> MEEPEEPADSGQSLVPVYIYSPEYVSMCDSLAKIPKRASMVHSLIEAYALHKQMRIVKPKVASMEEMATFHTDAYLQHLQKVSQEGDDDHPDSIEYGLGYDCPATEGIFDYAAAIGGATITAAQCLIDGMCKVAINWSGGWHHAKKDEASGFCYLNDAVLGILRLRRKFERILYVDLDLHHGDGVEDAFSFTSKVMTVSLHKFSPGFFPGTGDVSDVGLGKGRYYSVNVPIQDGIQDEKYYQICESVLKEVYQAFNPKAVVLQLGADTIAGDPMCSFNMTPVGIGKCLKYILQWQLATLILGGGGYNLANTARCWTYLTGVILGK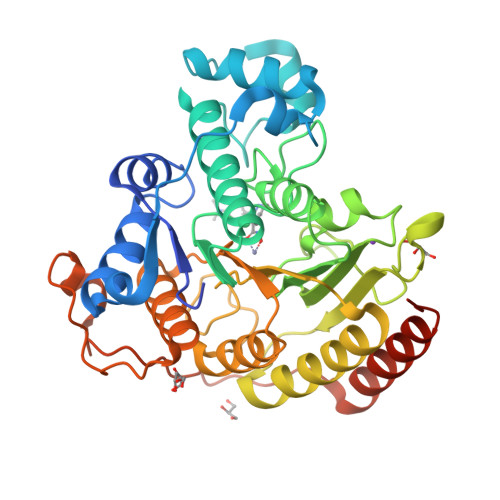TLSSEIPDREFFTAYGPDYVLEITPSCRPDRNEPHRIQQILNYIKGNLKHVVIEGRGSHHHHHH> SDCGLPPDVPNAQPALEGRTSFPEDTVITYKCEESFVKIPGEKDSVICLKGSQWSDIEEFCNRSCEVPTRLNSASLKQPYITQNYFPVGTVVEYECRPGYRREPSLSPKLTCLQNLKWSTAVEFCKKKSCPNPGEIRNGQIDVPGGILFGATISFSCNTGYKLFGSTSSFCLISGSSVQWSDPLPECREIYCP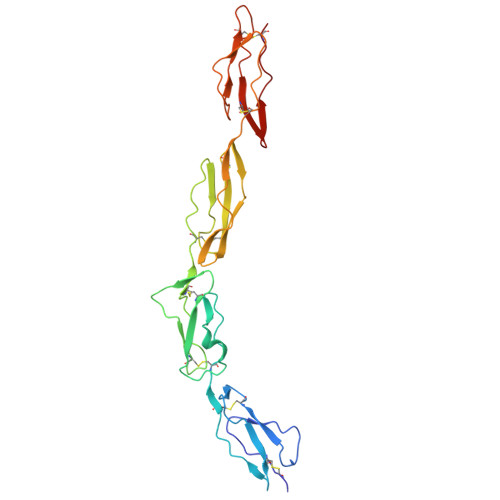APPQIDNGIIQGERDHYGYRQSVTYACNKGFTMIGEHSIYCTVNNDEGEWSGPPPECR> AGSVDTVSLYSGRGANMPFTIMEAESTSNATNGTKLTPNFKPGDYAGEASGRSSVYLDATGEYVEFTLTSPANAFVLRNAVAENTTGTVSIYADGVSKGKFNVSSKFSYLYATPSTLGRLGYDNAPGAGLTAYWLYEDAQLMLDQVYPAGTKI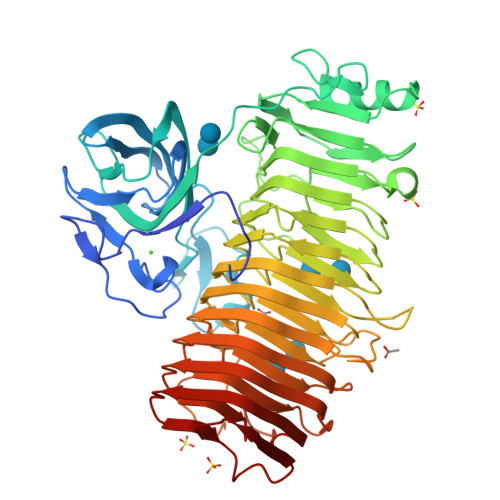KIQKDAGDVSWIYVDLLETENVAPPQANPDPTKYVAVSASKSIDQALTEFRQDNTKKGIYIPAGEWTINSKIFLYGRATEIVGAGPWYTKLVAPQSQSNTDVGFNISAAANGSTIRDLSAWGNYINRVDGPGKFIDGNGMQNVTVQNIWVEHFVCLYWGVNSSYNTFKNNRIKNTFADGINMTNGSSYNVIDNNYARGTGDASFALFSATDSGGSYNVGNKYTNLTATNVRRAAAFAVYGGSDNLFQNLYGADTLTYPGITISSYSFGYNTLGFGDQDTVIDGATLDRTGGDFWTSVGADDKINEYQNFGAIWIYGGDRAIKNILIKNVDINNPVYFGLMFQSMSPNNMVMQNIRVENVNINNPSRYGIKLVVRAEQGQGPAYGGASFTNVKVNNPGISAIYGEAQSPNFTVTRVSGNNW2-AZASQUALENE | C29 H51 N | 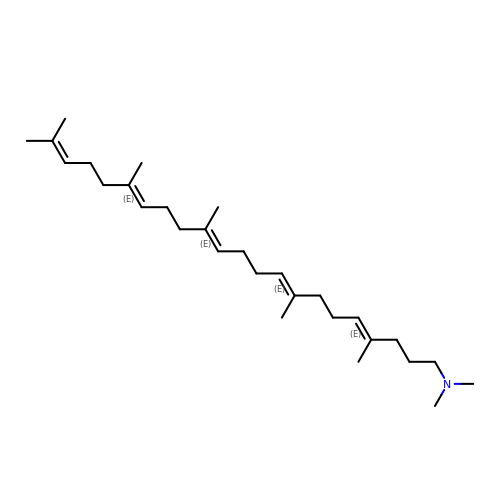OBYAAZRQFIVRJS-GUUMBNHASA-N> GPVCAEASDVYSPCMIASTPPAPFSDVTAVTFDLINGKITPVGDDNWNTHIYNPPIMNVLRTAA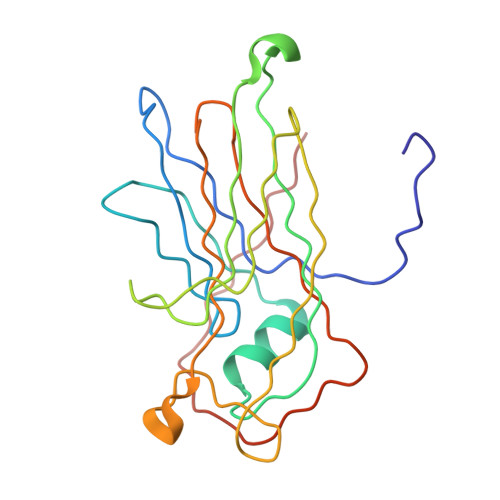WKSGTIHVQLNVRGAGVKRADWDGQVFVYLRQSMNPESYDARTFVISQPGSAMLNFSFDIIGPNSGFEFAESPWANQTTWYLECVATNPRQIQQFEVNMRFDPNFRVAGNILMPPFPLSTETPPL> TFPHERGNWATHVYVPYEAKEEFLDLLDVLLPHAQTYVPRLV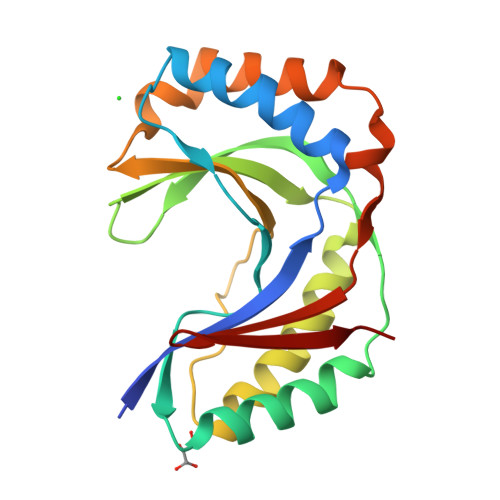RMKVFHLSLSQSVVLRHHWILPFVQALKARMTSFHRFFFTANQVKIYTNQEKTRTFIGLEVTSGHAQFLDLVSEVDRVMEEFNLTTFYQDPSFHLSLAWCVGDARLQLEGQCLQELQAIVDGFEDAEVLLRVHTEQVRCKSGNKFFSMPLK> MKPFLLGLLKCKRCSFMTKLILECEKAESNDVDTDDVKIFNKHMFTENGGERLKSLVNSLRDFHGRELSEQDISSFVENPGDDEKIKEFLFGIDVVEGSLRCDMCGLIYPIKGSIVETVDTVESK;> MDWYEPGEDTYTLMDALEREGLEMKIVLDLGT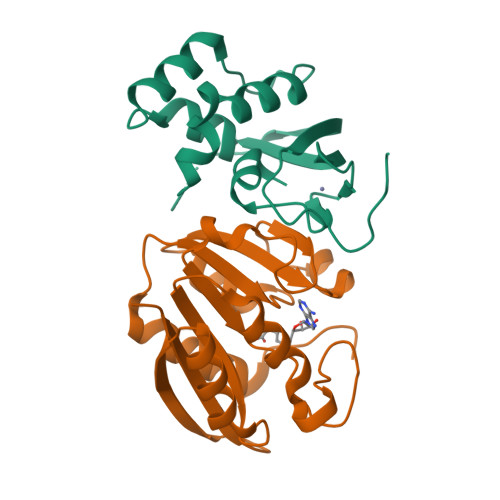STGVITEQLRKRNTVVSTDLNIRALESHRGGNLVRADLLCSINQESVDVVVFNPPYVPDTDDPIIGGGYLGREVIDRFVDAVTVGMLYLLVIEANRPKEVLARLEERGYGTRILKVRKILGETVYIIKGEKSHHHHHH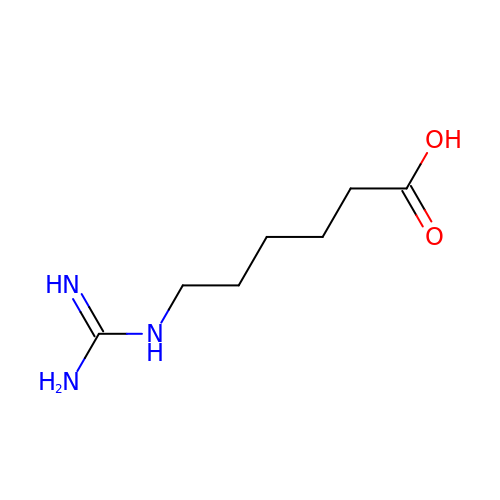6-carbamimidamidohexanoic acid | C7 H15 N3 O2 | NSDYIDKTTPXCRH-UHFFFAOYSA-N TDO and IDO are heme proteins that catalyze the oxidative cleavage of L-Trp, the first and rate-limiting step of the kynurenine pathway for L-Trp catabolism. TDOs are homo-tetrameric enzymes with 35–45 kD monomers and are well conserved from bacteria to humans. The hTDO monomer has an all α-helical structure, and the helices are named αA through αL, as in XcTDO. The heme is located at one end of this four-helical bundle, with the proximal His328 ligand coming from the C-terminal region of helix αJ.

To define the binding mode of O2 with respect to L-Trp and to obtain direct molecular insight into the catalytic mechanism, we prepared crystals of ferrous hTDO in complex with L-Trp under anaerobic conditions and then exposed them to an O2-saturated solution at room temperature. We observed a large change in the absorption spectrum of the crystal after overnight exposure to O2, indicating O2 binding and dioxygenation reaction. The final atomic model, at 2.5 Å resolution, has excellent agreement with the crystallographic data and the expected bond lengths, bond angles, and other geometric parameters. The crystallographic analysis revealed that the active sites of the four subunits of the hTDO tetramer are in different states in terms of the catalytic conversion of L-Trp, giving us several snapshots along the reaction coordinate. Clear electron density was observed for L-Trp and O2 in subunits A and B, allowing the definition of the relative regioorientation of the two substrates prior to the reaction for the first time. The O2 substrate is coordinated to the heme iron as the sixth ligand. The terminal oxygen atom is situated next to the plane of the L-Trp indole ring, close to its C2 (2.9 Å distance) and N1 (2.5 Å) atoms. The electron density in the active site of subunit C and subunit D is consistent with the product NFK, allowing us to define for the first time the binding mode of this product to TDO. The pyrrole ring of the Trp side chain has opened, but good electron density was observed only for the remaining six-membered ring and its N-formyl group, which is coordinated to the heme iron. The JK loop is ordered in subunit C but disordered in subunit D.

>[4x]MLPVEGSEEDKSQTGVNRASKGGLIYGNYLHLEKVLNAQELQSETKGNKIHDEHLFIITHQAYELWFKQILWELDSVREIFQNGHVRDERNMLKVVSRMHRVSVILKLLVQQFSILETMTALDFNDFREYLSPASGFQSLQFRLLENKIGVLQNMRVPYNRRHYRDNFKGEENELLLKSEQEKTLLELVEAWLERTPGLEPHGFNFWGKLEKNITRGLEEEFIRIQAKEESEEKEEQVAEFQKQKEVLLSLFDEKRHEHLLSKGERRLSYRALQGALMIYFYREEPRFQVPFQLLTSLMDIDSLMTKWRYNHVCMVHRMLGSKAGTGGSSGYHYLRSTVSDRYKVFVDLFNLSTYLIPRHWIPKMNPTIHKFLEHHHHHH N-(PYRAZIN-2-YLCARBONYL)LEUCYLISOLEUCYL-N~1~-{1-[2-({1-CARBOXY-2-[4-(PHOSPHONOOXY)PHENYL]ETHYL}AMINO)-1,1-DIHYDROXY-2-OXOETHYL]BUT-3-ENYL}-3-CYCLOHEXYLALANINAMIDE 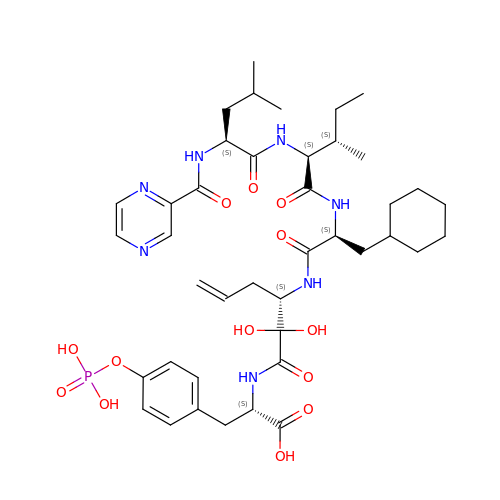| C41 H60 N7 O13 P | NANINTGNSYDVAR-PBWGIQFFSA-N>GPVDVKLEFVLYRKNVTLAELEAMGQQQLLSLPTNAELNVEIMANGVLLGNGELVQMNDTLGVEIHEW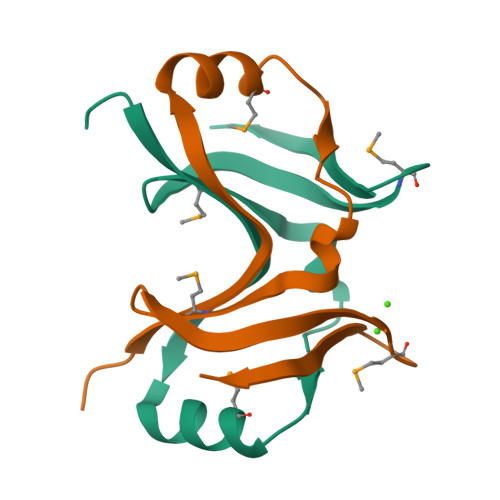LS[2x]> MVPISPIETVPVKLKPGMDGPKVKQWPLTEEKIKALVEICTEMEKEGKISKIGPENPYNTPVFAIKKKDSTKWRKLVDFRELNKRTQDFWEVQLGIPHPAGLKKKKSVTVLDVGDAYFSVPLDEDFRKYTAFTIPSINNETPGIRYQYNVLPQGWKGSPAIFQSSMTKILEPFAAQNPDIVIYQYMDDLLVGSDLEIGQHRTKIEELRQHLLRWGLTTPDKKHQKEPPFLWMGYELHPDKWTVQPIVLPEKDSWTVNDIQKLVGKLNWASQIYPGIKVRQLSKLLRGTKALTEVIPLTEEAELELAENREILKEPVHGVYYDPSKDLIAEIQKQGQGQWTYQIYQEPFKNLKTGKYARMRGAHTNDVKQLTEAVQKITTESIVIWGKTPKFKLPIQKETWETWWTEYWQATWIPEWEFVNTPPLVKLWYQLEKEPIVGAET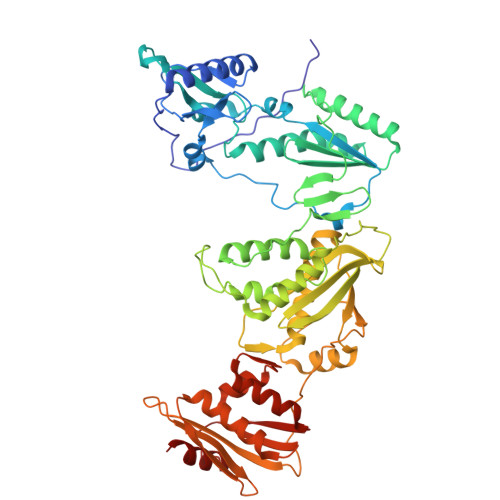FYVDGAANRETKLGKAGYVTNKGRQKVVPLTNTTNQKTELQAIYLALQDSGLEVNIVTDSQYALGIIQAQPDKSESELVNQIIEQLIKKEKVYLAWVPAHKGIGGNEQVDKLVSAG>MEEKRLSAKKGLPPGTLVYTGKYRED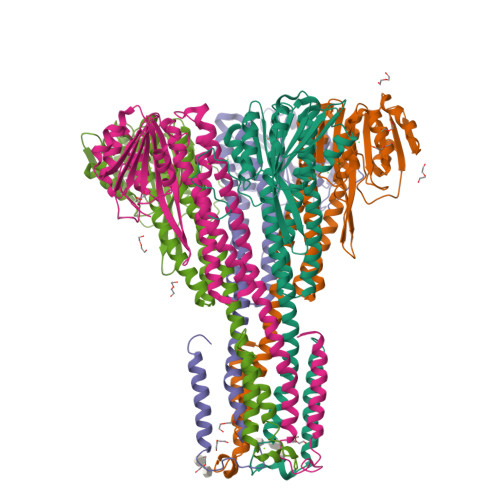FEIEVMNYSIEEFREFKTTDVESVLPFRDSSTPTWINITGIHRTDVVQRVGEFFGIHPLVLEDILNVHQRPKVEFFENYVFIVLKMFTYDKNLHELESEQVSLILTKNCVLMFQEKIGDVFDPVRERIRYNRGIIRKKRADYLLYSLIDALVDDYFVLLEKIDDEIDVLEEEVLERPEKETVQRTHQLKRNLVELRKTIWPLREVLSSLYRDVPPLIEKETVPYFRDVYDHTIQIADTVETFRDIVSGLLDVYLSSVSNKTNEVMKVLTIIATIFMPLTFIAGIYGMNFEYMPELRWKWGYPVVLAVMGVIAVIMVVYFKKKKWL[10x]> SMARIGDLDAARPAPEAVPGDMVRIPGGTFLQGSPERTLDWLDREGQAFPRDWFTDETPQIPVTLPDYLIDRHQVTVAQFAAFVSRTGYVTSAERAGGSMVYGEQYWEIREGACWHRPAGYGSGIRGRDDHPVVHISFADAEAYARWAGRRLPTESEWERAATGPSYRLWPWGDTWDSRNANTAEHTAGALGDLDAWRTWWGAIHAVQGPMPQTTPVGAFSPRGDSVDGCADMTG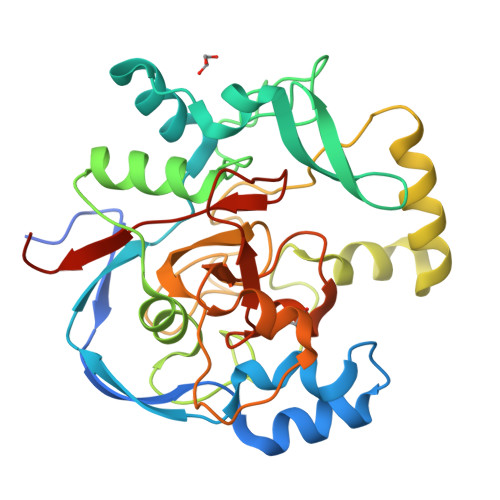NVYEWTSTLAHLYSPATRCDPTIHLVMGRSRVIRGGSWMNFRYQVRCAERLYGDPTGWSNFALGFRCARDVTAVPHVDDNGR> HMAALDSLSLFTSLGLSEQKARETLKNSALSAQLREAATQAQQTLGSTIDKATGILLHGLASRLRDTRRLSFLVSYIASKKIHTEPQLSAALEYVRSHPLDPIDTVDFERECGVGVIVTPEQIEEAVEAAINRHRPQLLVERYHFNMGLLMGEARAVLKWADGKMIKNEVDMQVLHLLGPKLEADLEKKFKVAKARLEE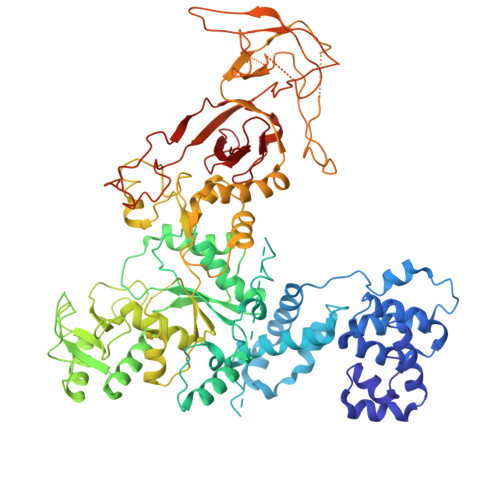TDRRTAKDVVENGETADQTLSLMEQLRGEALKFHKPGENYKTPGYVVTPHTMNLLKQHLEITGGQVRTRFPPEPNGILHIGHAKAINFNFGYAKANNGICFLRFDDTNPEKEEAKFFTAICDMVAWLGYTPYKVTYASDYFDQLYAWAVELIRRGLAYVCHQRGEELKGHNTLPSPWRDRPMEESLLLFEAMRKGKFSEGEATLRMKLVMEDGKMDPVAYRVKYTPHHRTGDKWCIYPTYDYTHCLCDSIEHITHSLCTKEFQARRSSYFWLCNALDVYCPVQWEYGRLNLHYAVVSKRKILQLVATGAVRDWDDPRLFTLTALRRRGFPPEAINNFCARVGVTVAQTTMEPHLLEACVRDVLNDTAPRAMAVLESLRVIITNFPAAKSLDIQVPNFPADETKGFHQVPFAPIVFIERTDFKEEPEPGFKRLAWGQPVGLRHTGYVIELQHVVKGPSGCVESLEVTCRRADAGEKPKAFIHWVSQPLMCEVRLYERLFQHKNPEDPTEVPGGFLSDLNLASLHVVDAALVDCSVALAKPFDKFQFERLGYFSVDPDSHQGKLVFNRTVTLKEDPGKV Silicatein is the first discovered enzymatically active multifunctional protein that catalyzes the polymerization of biogenic silica and is key to its subsequent condensation and shaping. Using a close homology to the cathepsin protein family—sequence identity between silicatein-α in T. aurantium and metazoan cathepsin L is 52%—silicatein’s mechanism of catalysis was modeled. It is suggested that, analogous to the hydrolysis of peptide bonds in the cysteine proteases by cathepsin, a catalytic triad composed of Ser, His, and Asn (a serine protease) is key to the polycondensation of silicic acid by silicatein-α. The filaments in demosponges were demonstrated to be perfect slender protein crystals, and their branching on well-defined crystallographic planes of that crystal was shown to be responsible for the high spatial regularity and symmetry of the spicules.

The tertiary structure of silicatein-α, occurring in a crystalline form in vivo, was measured in situ by serial crystallography and realized at a protein crystallography beamline at a synchrotron. In this work, a total of 3,608 individual diffraction snapshots were collected in cryogenic conditions from 90 different needle-like spicules extracted from the sponge T. aurantium. In each spicule, a rectangular beam of 30 µm × 10 µm was rastered along the axial filament to avoid measuring a previously damaged area. These data were sufficient to generate a complete dataset with a resolution of 2.4 Å. Using the known sequence of the most abundant isoform of silicatein, silicatein-α, a well-defined electron density was obtained allowing the reconstruction of a continuous protein model from Pro3 to the C-terminal residue Leu218 (except of loop Ser175 to Gln178). Surprisingly, these data reveal that the postulated active site of the protein—the catalytic triad of Ser26, His165, and Asn185—is in an inactive mode. The distance between the hydroxyl group of Ser26 and the imidazole ring of His165 is 3.6 Å, too long to allow catalytic conformation. It can be hypothesized that a rotation of the Ser26 side chain into another favorable conformation (a distance of 2.9 Å to the imidazole ring of His165) leads to activation of the enzymatic activity of silicatein, which is also supported by an additional hydrogen bond network including Gln20 and Ser186. However, in its crystalline form, in the axial filament inside the spicule, the enzymatic activity of the protein is switched off. To form the axial filament, the silicatein molecules are packed into a single slender crystal with six proteins in a single hexagonal unit cell belonging to the symmetry group P3121 with a = 5.96 nm and c = 11.63 nm. Remarkably, the modeled images obtained parallel to the c-axis and the a-axis fully agree with the experimental TEM measurements.

> AYPETVDWRTKGAVTGIKSQGDCGASYAFSAMGALEGINALATGKLTYLSEQNIIDCSVPYGNHGCKGGNMYVAFLYVVANEGVDDGGSYPFRGKQSSCTYQEQYRGASMSGSVQINSGSESDLEAAVANVGPVAVAIDGESNAFRFYYSGVYDSSRCSSSSLNHAMVITGYGISNNQEYWLAKNSWGENWGELGYVKMARNKYNQCGIASDASYPTL>MFHGKHPGGLSERGRALLLEGGKALGLDLKPHLEAFSRLYALLQEASGKVNLTALRGEEEVVVKHFLDSLTLLRLPLWQGPLRVLDLGTGAGFPGLPLKIVRPELELVLVDATRKKVAFVERAIEVLGLKGARALWGRAEVLAREAGHREAYARAVARAVAPLCVLSELLLPFLEVGGAAVAMKGPRVEEELAPLPPALERLGGRLGEVLALQLPLSGEARHLVVLEKTAPTPPAYPRRP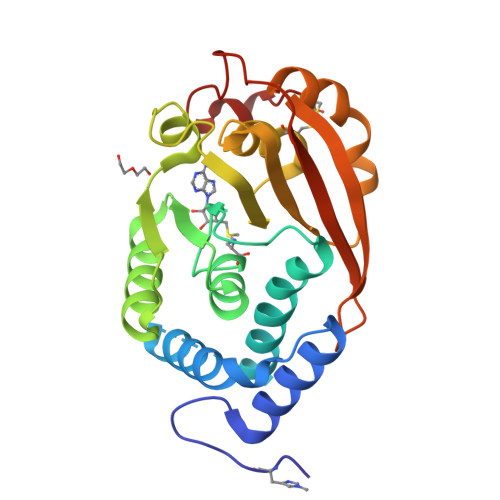GVPERHPLC[2x]>MAHSSATAGPQADFSGEIAEL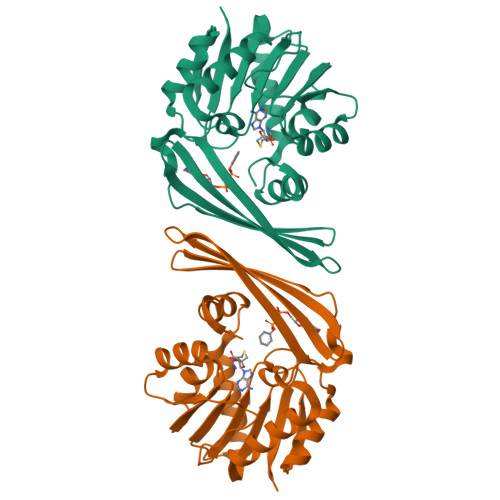YDLVHQGKGKDYHREAADLAALVRRHSPKAASLLDVACGTGMHLRHLADSFGTVEGLELSADMLAIARRRNPDAVLHHGDMRDFSLGRRFSAVTCMFSSIGHLAGQAELDAALERFAAHVLPDGVVVVEPWWFPENFTPGYVAAGTVEAGGTTVTRVSHSSREGEATRIEVHYLVAGPDRGITHHEESHRITLFTREQYERAFTAAGLSVEFMPGGPSGRGLFTGLPGAKGETRLEHHHHHH[4x]>MWKRSEQMKIKSGKCNMAAAMETEQLGVEIFETADCEENIESQDRPKLEPFYVERYSWSQLKKLLADTRKYHGYMMAKAPHDFMFVKRNDPDGPHSDRIYYLAMSGENRENTLFYSEIPKTINRAAVLMLSWKPLLDLFQATLDYGMYSREEELLRERKRIGTVGIASYDYHQGSGTFLFQAGSGIYHVKDGGPQGFTQQPLRPNLVETSCPNIRMDPKLCPADPDWIAFIHSNDIWISNIVTREERRLTYVHNELANMEEDARSAGVATFVLQEEFDRYSGYWWCPKAETTPSGGKILRILYEENDESEVEIIHVTSPMLETRRADSFRYPKTGTANPKVTFKMSEIMIDAEGRIIDVIDKELIQPFEILFEGVEYIARAGWTPEGKYAWSILLDRSQTRLQIVLISPELFIPVEDDVMERQRLIESVPDSVTPLIIYEETTDIWINIHDIFHVFPQSHEEEIEFIFASECKTGFRHLYKITSILKESKYKRSSGGLPAPSDFKCPIKEEIAITSGEWEVLGRHGSNIQVDEVRRLVYFEGTKDSPLEHHLYVVSYVNPGEVTRLTDRGYSHSCCISQHCDFFISKYSNQKNPHCVSLYKLSSPEDDPTCKTKEFWATILDSAGPLPDYTPPEIFSFESTTGFTLYGMLYKPHDLQPGKKYPTVLFIYGGPQVQLVNNRFKGVKYFRLNTLASLGYVVVVIDNRGSCHRGLKFEGAFKYKMGQIEIDDQVEGLQYLASRYDFIDLDRVGIHGWSYGGYLSLMALMQRSDIFRVAIAGAPVTLWIFYDTGYTERYM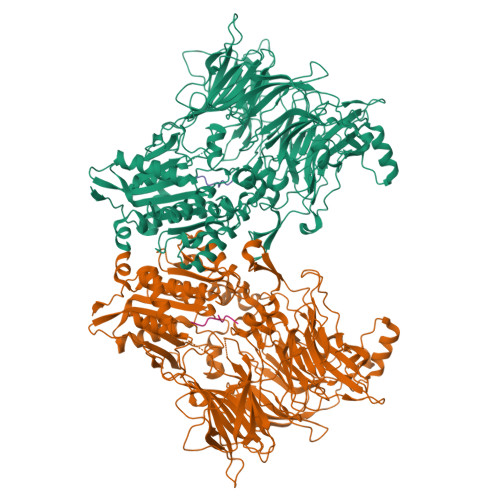GHPDQNEQGYYLGSVAMQAEKFPSEPNRLLLLHGFLDENVHFAHTSILLSFLVRAGKPYDLQIYPQERHSIRVPESGEHYELHLLHYLQENLGSRIAALKVI[6x];>SLRFLYEG[6x]> EDEDGDYEELVLALRSEEDGLAEAPEHGTTATFHRCAKDPWRLPGTYVVVLKEETHLSQSERTARRLQAQAARRGYLTKILHVFHGLLPGFLVKMSGDLLELALKLPHVDYIEEDSSVFAQ;> SIPWNLERITPPRYRADEYQPPDGGSLVEVYLLDTSIQSDHREIEGRVMVTDFENVPEEDGTRFHRQASKCDSHGTHLAGVVSGRDAGVAKGASMRSLRVLNCQGKGTVSGTLIGLEFIRKSQLVQPVGPLVVLLPLAGGYSRVLNAACQRLARAGVVLVTAAGNFRDDACLYSPASAPEVITVGATNAQDQPV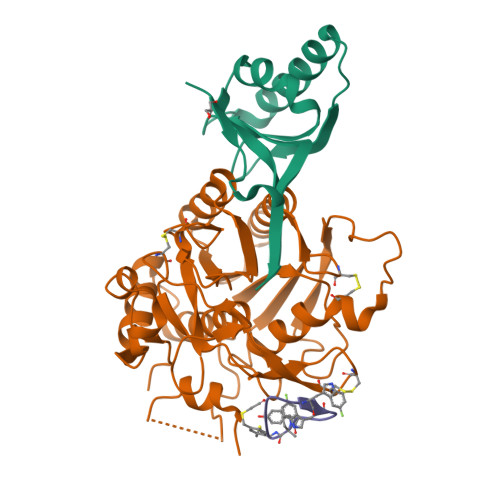TLGTLGTNFGRCVDLFAPGEDIIGASSDCSTCFVSQSGTSQAAAHVAGIAAMMLSAEPELTLAELRQRLIHFSAKDVINEAWFPEDQRVLTPNLVAALPPSTHGAGNSHHHHHH>HHHHHHMRVSFMVAMDENRVIGKDNNLPWRLPSELQYVKKTTMGHPLIMGRKNY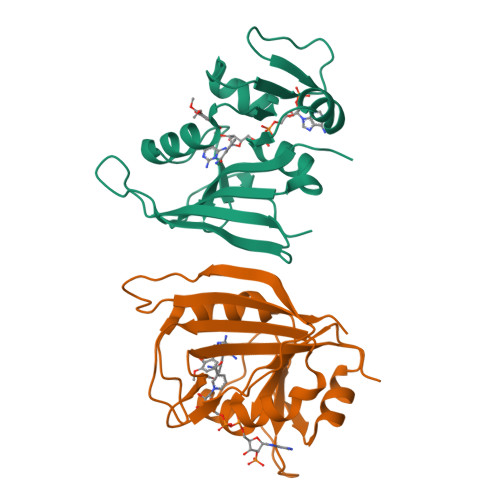EAIGRPLPGRRNIIVTRNEGYHVEGCEVAHSVEEVFELCKNEEEIFIFGGAQIYDLFLPYVDKLYITKIHHAFEGDTFFPEMDMTNWKEVFVEKGLTDEKNPYTYYYHVYEKQQ[2x]> MGSSHHHHHHSSGLVPRGSHMSSDSSVAASAQPPIAAKKPHRVTLGYVEGEDRGPNPMNPPRYREDPYFWMRDDDRKDPAVIEHLNKEKVYFQARSADIAQLRDDIYAEHISHINEDDMSAPYVYGKYRYYTREVKGKPYKIYCRVFTDKEPGDVAAEEVIIDVNQVAEGKAFCD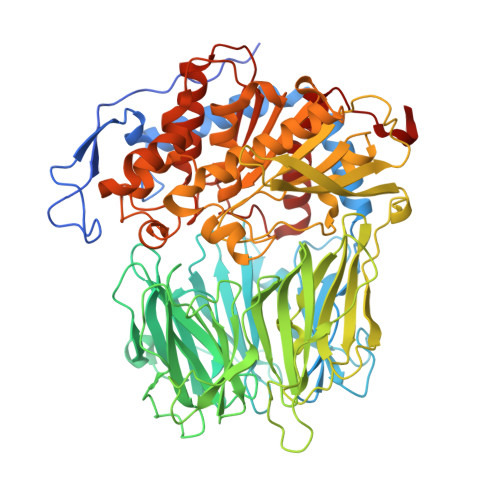VMEVKPAPPEHDLVAFSVDMSGNEVYTIEFKRISDPSQTIADKVSGTNGEIVWGPDHTSLFYVTKDETLRENKVWRHVMGKLQSEDVCLYEEHNPLFSAFMYKAADTNTLCIGSQSPETAEVHLLDLRKGNAHNTLEIVRPREKGVRYDVQMHGTSHLVILTNEGGAVNHKLLIAPRGQPSDWSHVLVDHSEDVFMESIAVRSNYLVVAGRRAGLTRIWTMMADSQDGVFKAGTGLREVVMEEPIFTVHLVESQMLEYEEPTFRMEYSSLATPNTWFDVSPQDHSRTAVKVREVGGGFDAANYKVERRFATAPDQTKIPLSVVYHKDLDMSQPQPCMLYGYGSYGLSMDPQFSIQHLPYCDRGMIFAIAHIRGGSELGRAWYEIGAKYLTKRNTFSDFIAAAEFLVNAKLTTPSQLACEGRSAGGLLMGAVLNMRPDLFKVALAGVPFVDVMTTMCDPSIPLTTGEWEEWGNPNEYKYYDYMLSYSPMDNVRAQEYPNIMVQCGLHDPRVAYWEPAKWVSKLRECKTDNNEILLNIDMESGHFSAKDRYKFWKESAIQQAFVCKHLKSTVRLLVRR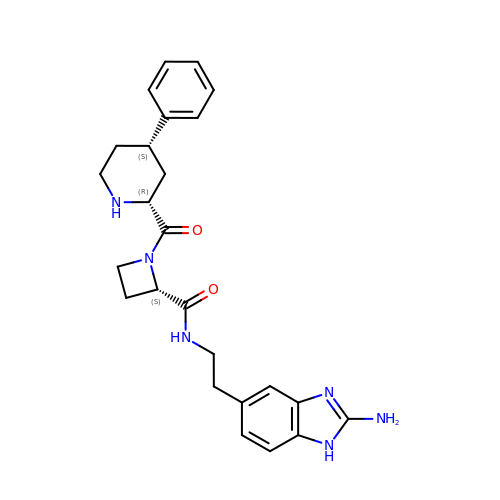(2S)-N-[2-(2-amino-1H-1,3-benzimidazol-5-yl)ethyl]-1-[(2R,4S)-4-phenylpiperidine-2-carbonyl]azetidine-2-carboxamide | C25 H30 N6 O2 | JAQKIQJBWFVAMC-BWAGFHJFSA-N>MEPRPTAPSSGAPGLAGVGETPSAAALAAARVELPGTAVPSVPEDAAPASRDGGGVRDEGPAAAGDGLGRPLGPTPSQSRFQVDLVSENAGRAAAAAAAAAAAAAAAGAGAGAKQTPADGEASGESEPAKGSEEAKGRFRVNFVDPAASSSAEDSLSDAAGVGVDGPNVSFQNGGDTVLSEGSSLHSGGGGGSGHHQHYYYDTHTNTYYLRTFGHNTMDAVPRIDHYRHTAAQLGEKLLRPSLAELHDELEKEPFEDGFANGEESTPTRDAVVTYTAESKGVVKFGWIKGVLVRCMLNIWGVMLFIRLSWIVGQAGIGLSVLVIMMATVVTTITGLSTSAIATNGFVRGGGAYYLISRS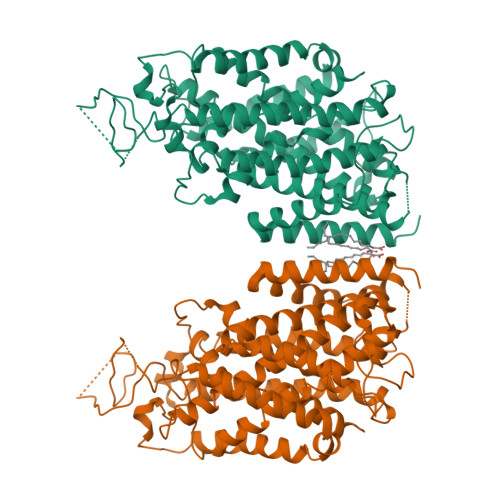LGPEFGGAIGLIFAFANAVAVAMYVVGFAETVVELLKEHSILMIDEINDIRIIGAITVVILLGISVAGMEWEAKAQIVLLVILLLAIGDFVIGTFIPLESKKPKGFFGYKSEIFNENFGPDFREEETFFSVFAIFFPAATGILAGANISGDLADPQSAIPKGTLLAILITTLVYVGIAVSVGSCVVRDATGNVNDTIVTELTNCTSAACKLNFDFSSCESSPCSYGLMNNFQVMSMVSGFTPLISAGIFSATLSSALASLVSAPKIFQALCKDNIYPAFQMFAKGYGKNNEPLRGYILTFLIALGFILIAELNVIAPIISNFFLASYALINFSVFHASLAKSPGWRPAFKYYNMWISLLGAILCCIVMFVINWWAALLTYVIVLGLYIYVTYKKPDVNWGSSTQALTYLNALQHSIRLSGVEDHVKNFRPQCLVMTGAPNSRPALLHLVHDFTKNVGLMICGHVHMGPRRQAMKEMSIDQAKYQRWLIKNKMKAFYAPVHADDLREGAQYLMQAAGLGRMKPNTLVLGFKKDWLQADMRDVDMYINLFHDAFDIQYGVVVIRLKEGLDISHLQGQEELLSSQEKSPGTKDVVVSVEYSKKSDLDTSKPLSEKPITHKVEEEDGKTATQPLLKKESKGPIVPLNVADQKLLEASTQFQKKQGKNTIDVWWLFDDGGLTLLIPYLLTTKKKWKDCKIRVFIGGKINRIDHDRRAMATLLSKFRIDFSDIMVLGDINTKPKKENIIAFEEIIEPYRLHEDDKEQDIADKMKEDEPWRITDNELELYKTKTYRQIRLNELLKEHSSTANIIVMSLPVARKGAVSSALYMAWLEALSKDLPPILLVRGNHQSVLTFYS[2x]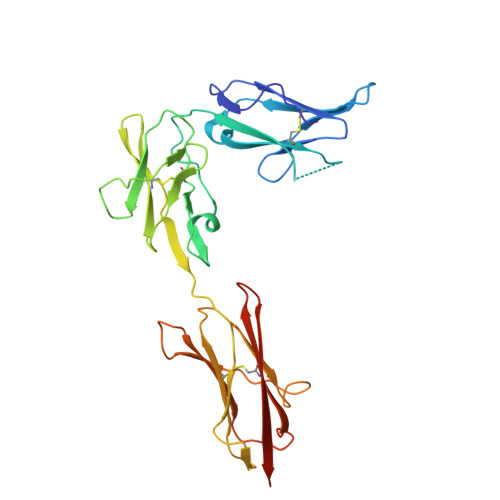> LVVTPPGPELVLNVSSTFVLTCSGSAPVVWERMSQEPPQEMAKAQDGTFSSVLTLTNLTGLDTGEYFCTHNDSRGLETDERKRLYIFVPDPTVGFLPNDAEELFIFLTEITEITIPCRVTDPQLVVTLHEKKGDVALPVPYDHQRGFSGIFEDRSYICKTTIGDREVDSDAYYVYRLQVSSINVSVNAVQTVVRQGENITLMCIVIGNEVVNFEWTYPRKESGRLVEPVTDFLLDMPYHIRSILHIPSAELEDSGTYTCNVTESVNDHQDEKAINITVVESGHHHHHHH>TVVEEPVDITPYLDQLDESLRDKVLQLQKGSDTEAQCEVMQEIVDQVLEEDFDSEQLSVLASCLQELFKAHFRGEVLPEEITEESLEESVGKPLYLIFRNLCQMQEDNSSFSLLLDLLSELYQKQPKIGYHLLYYLRASKAAAGKMNLYESFAQATQLGDLHTCLMMDMKACQEDDVRLLCHLTPSIYTEFPDETLRSGELLNMIVAVIDSAQLQELVCHVMMGNLVMFRKDSVLNILIQSLDWETFEQYCAWQLFLAHNIPLETIIPILQHLKYKEHPEALSCLLLQLRREKPSEEMVKMVLSRPCHPDDQFTTSILRHWCMKHDELLAEHIKSLLIKNNSLPRKRQSLRSSSSKLAQLTLEQILEHLDNLRLNLTNTKQNFFSQTPILQALQHVQASCDEAHKMKFSDLFSLAEEYEDSSTKPPKSRRKAALSS[2x];> MHCRSHEEVNTELKAQIMKEIRKPGRKYERIFTLLKHVQGSLQTRLIFLQNVIKEASRFKKRMLIEQLENFLDEIHRRANQINHINSN

SOSS1 is a single-stranded DNA (ssDNA)-binding protein complex that plays a critical role in double-strand DNA break (DSB) repair. SOSS1 consists of three subunits: INTS3, SOSSC, and hSSB1, with INTS3 serving as a scaffold to stabilize this complex. Moreover, the integrator complex subunit 6 (INTS6) participates in the DNA damage response through direct binding to INTS3, but how INTS3 interacts with INTS6, thereby impacting DSB repair, is not clear. In response to DSBs, INTS6 is recruited to DSBs by directly interacting with INTS3c.

To clarify the molecular mechanism underlying the assembly of the INTS3/INTS6 complex in DSB repair, we crystallized and determined the crystal structure of the INTS3c (residues 560–905, 915–995)/INTS6c (residues 800–887) complex. The structure of the INTS3c/INTS6c complex reveals an all α-helical assembly resembling the shape of a “butterfly”, with the INTS3c dimer forming the wings and one INTS6c subunit near the two-fold axis of the dimer interface making the body of the butterfly. The molar ratio between INTS3c and INTS6c is 2:1. INTS3c adopts a right-handed super-helical structure with 20 helices, in which each helix is paired with its neighboring helix to form an antiparallel helix pair. INTS6c contains four α-helices and interacts with INTS3c via two loops between α1−α2 and α3−α4. Two INTS3c protomers form a symmetrical dimer wherein two protomers are related by a non-crystallographic two-fold axis. Analysis of the dimer interface using Protein Interfaces, Surfaces, and Assemblies webserver (PISA)22 revealed a buried surface area of ~3400.0 Å2. The bulk of the hydrophobic core consists of Leu773, Phe806, Tyr809, and Leu846 from both chains of the dimer. The core of the interface is hydrophobic in nature with Pro823 and Phe858 of INTS6c juxtaposed against Phe806 from the two subunits of INTS3c. The interaction is further augmented by salt bridges between Lys859 of INTS6c and Glu839 of INTS3c, Arg825 of INTS6c and Glu804 and Glu807 of INTS3c, and Arg857 of INTS6c and Asp769 of INTS3c.>[2x]PFELPALPYPYDALEPHIDKETMNIHHTKHHNTYVTNLNAALEGHPDLQNKSLEELLSNLEALPESIRTAVRNNGGGHANHSLFWTILSPNGGGEPTG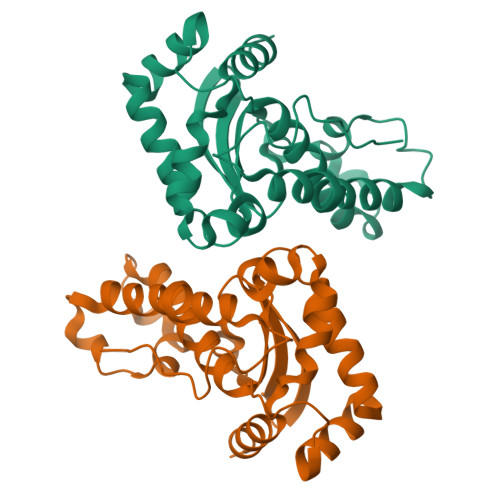ELADAINKKFGSFTAFKDEFSKAAAGRFGSGWAWLVVNNGELEITSTPNQDSPIMEGKTPILGLDVWEHAYYLKYQNRRPEYIAAFWNVVNWDEVAKRYSEAKA>MAHHHHHHMLDINLFREYKGGNPEIIRESQRRRFADVTLVDKVIELDEVWRATIGKLNHIKSFTGIISKEVGNRMKNKVPLGDDLELPKEVTDDVYALFTKEALEQGSLAKLNTNQLKKLSTYITEVHIKNSEEEVKQKEKERDDVLLQIGNIVHETVVVSDNEDNNGIVRMVGNPRPKVDPETGYKCLKHIDIMRKLGGLATEEGTQVGGGRGYFLLGDLVRMNLALQNYAIDFLAKKGYMPIYTPFFMTKEQMKKVAQLSQFDEELYTVTGEGEDKYLIATSEQPIAAFHLEKRFDESELPIKYCGMSTCFRKEVGAHGKDTLGIFRVHQFEKIEQFVVTSPKDNKSWEMFDEMIGNSEAFYQSLGIPYRVVNIVSGALNNAAAKKFDLEAWFPGA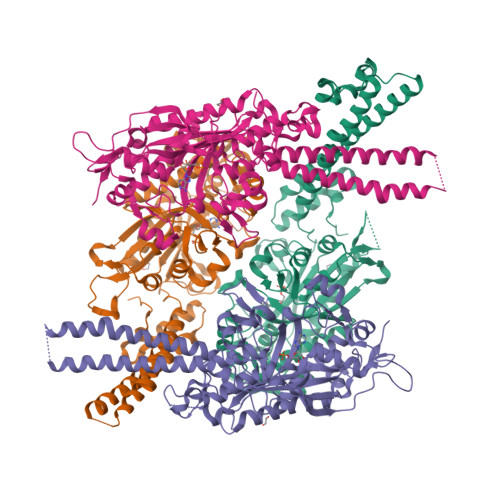DEGNEYRELVSCSNCTDYQTRRLEVKYGKSKKQGSEVEFCHMLNSTLTATSRTLCCIVENYQTPEGVNVPEVLQPYMGGTKFIKFKN[3x]>[4x]MSRRLRRTKIVTTLGPATDRDNNLEKVIAAGANVVRMNFSHGSPEDHKMRADKVREIAAKLGRHVAILGDLQGPKIRVSTFKEGKVFLNIGDK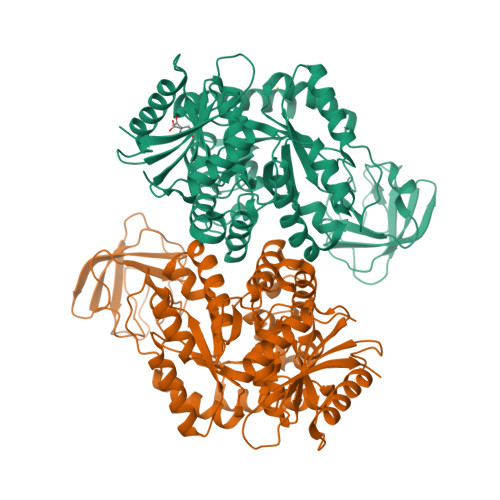FLLDANLGKGEGDKEKVGIDYKGLPADVVPGDILLLDDGRVQLKVLEVQGMKVFTEVTVGGPLSNNKGINKLGGGLSAEALTEKDKADIKTAALIGVDYLAVSFPRCGEDLNYARRLARDAGCDAKIVAKVERAEAVCSQDAMDDIILASDVVMVARGDLGVEIGDPELVGIQKALIRRARQLNRAVITATQMMESMITNPMPTRAEVMDVANAVLDGTDAVMLSAETAAGQYPSETVAAMARVCLGAEKIPSINVSKHRLDVQFDNVEEAIAMSAMYAANHLKGVTAIITMTESGRTALMTSRISSGLPIFAMSRHERTLNLTALYRGVTPVHFDSANDGVAAASEAVNLLRDKGYLMSGDLVIVTQGDVMSTVGSTNTTRILTVEALGHHHHHH1-[2-[5-[AMINO(IMINO)METHYL]-2-HYDROXYPHENOXY]-6-[3-(4,5-DIHYDRO-1-METHYL-1H-IMIDAZOL-2-YL)PHENOXY] PYRIDIN-4-YL]PIPERIDINE-3-CARBOXYLIC ACID | 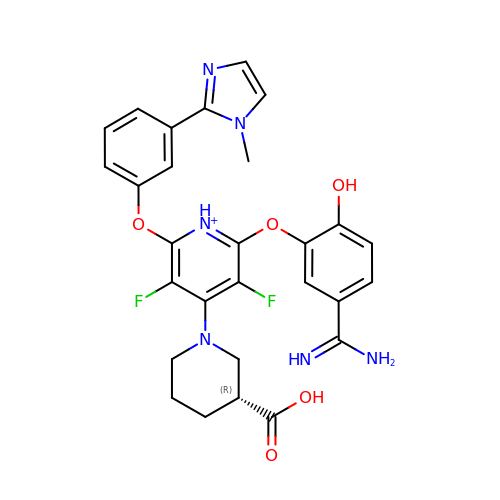C28 H27 F2 N6 O5 | PSJQZXADHMZXED-QGZVFWFLSA-O> MNARSTGQHPARYPGAAAGEPTLDSWQEPPHNRWAFAHLGEMVPSAAVSRRPVNAPGHALVRLGAIAAQLPDLEQRLEQTYTDAFLVLRGTEVVAEYYRAGFAPDD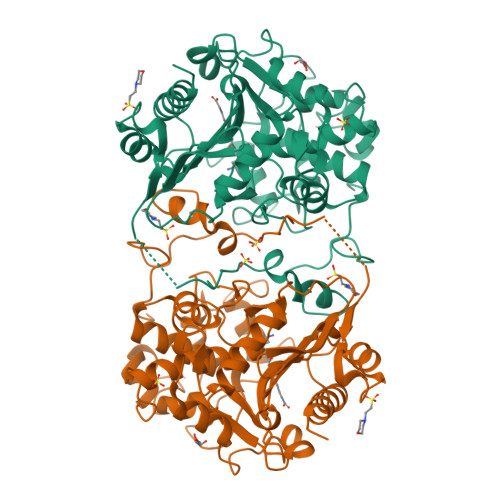RHLLMAVSKSLCGTVVGVLVDEGRIDPAQPVTEYVPELAGSVYDGPSVLQVLDMQISIDYNEDYVDPASEVQTHGRSAGWSTRRHGDPADTYEFLTTLRGDGSTGEFQYCSANTDVLAWIVERVTGLRYVEALSTYLWAKLDADRDATITVDTTGFGCAHGGVSCTARDLARVGRMMLDGGVAPRGRVVSEDWVRRVLAGGSHEAMTDKGFTNTFPDGSYTRQWWCTGNERANVSGIGIHGQNLWLDPLTDSVIVKLSSWPDPYTEHWHRLQNGILLDVSRALDAV> GNPIHDRTSDYHKYLKVKQGDSDLFKLTVSDKRYIWYNPDPKERDSYECGEIVSETSDSFTFKTVDGQDRQVKKDDANQRNPIKFDGVEDMSELSYLNEPAVFHNLRVRYNQDLIYTYSGLFLVAVNPFKRIPIYTQEMVDIFKGRRRNEVAPHIFAISDVAYRSMLDDRQNQSLLITGESGAGKTENTKKVIQYLASVAGRNQANGSGVLEQQILQANPILEAFGNAKTTRNNNASRFGKFIEIQFNSAGFISGASIQSYLLEKSRVVFQSETERNYHIFYQLLAGATAEEKKALHLAGPESFNYLNQSGCVDIKGVSDSEEFKITRQAMDIVGFSQEEQMSIFKIIAGILHLGNIKFEKGAGEGAVLKDKTALNAASTVFGVNPSVLEKALMEPRILAGRDLVAQHLNVEKSSSSRDALVKALYGRLFLWLVKKINNVLCQERKAYFIGVLDISGFEIFKVNSFEQLCINYTNEKLQQFFNHHMFKLEQEEYLKEKINWTFIDFGLDSQATIDLIDGRQPPGILALLDEQSVFPNATDNTLITKLHSHFSKKNAKYEEPRFSKTEFGVTHYAGQVMYEIQDWLEKNKDPLQQDLELCFKDSSDNVVTKLFNDPNIASRAKKGANFITVAAQYKEQLASLMATLETTNPHFVRCIIPNNKQLPAKLEDKVVLDQLRCNGVLEGIRITRKGFPNRIIYADFVKRYYLLAPNVPRDAEDSQKATDAVLKHLNIDPEQYRFGITKIFFRAG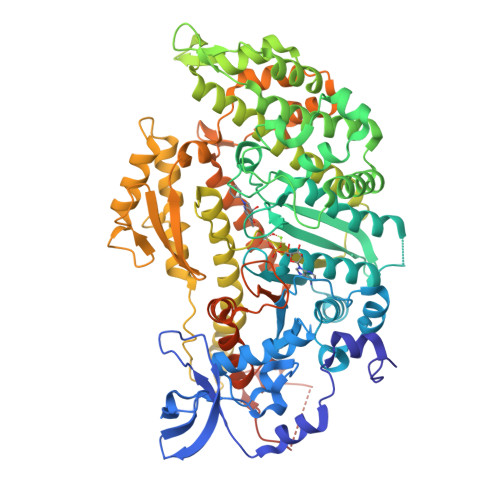QLARIEEARELPN> MSLSFCGNNISSYNIYHGVLQNPCFVDALNLVPHVFLLFITFPILFIGWGSQSSKVQIHHNTWLHFPGHNLRWILTFALLFVHVCEIAEGIVSDSQRASRHLHLFMPAVMGFVATTTSIVYYHNIETSNFPKLLLALFLYWVMAFITKTIKLVKYWQLGWGMSDLRFCITGVMVILNGLLMAVEINVIRVRRYVFFMNPQKVKPPEDLQDLGVRFLQPFVNLLSKATYWWMNTLIISAHRKPIDLKAIGKLPIAMRAVTNYVCLKEAYEEQKKKAADHPNRTPSIWLAMYRAFGRPILLSSTFRYLADLLGFAGPLCISGIVQRVNEPKNNTTRFSETLSSKEFLENAHVLAVLLFLALILQRTFLQASYYVTIETGINLRGALLAMIYNKILRLSTSNLSMGEMTLGQINNLVAIETNQLMWFLFLCPNLWAMPVQIIMGVILLYNLLGSSALVGAAVIVLLAPIQYFIATKLAEAQKSTLDYSTERLKKTNEILKGIKLLKLYAWEHIFCKSVEETRMKELSSLKTFALYTSLSIFMNAAIPIAAVLATFVTHAYASGNNLKPAEAFASLSLFHILVTPLFLLSTVVRFAVKAIISVQKLNEFLLSDEIGEDSWRTGEGTLPFESCKKHTGVQSKPINRKQPGRYHLDNYEQARRLRPAETEDVAIKVTNGYFSWGSGLATLSNIDIRIPTGQLTMIVGQVGCGKSSLLLAILGEMQTLEGKVYWNNVNESEPSFEATRSRSRYSVAYAAQKPWLLNATVEENITFGSSFNRQRYKAVTDACSLQPDIDLLPFGDQTEIGERGINLSGGQRQRICVARALYQNTNIVFLDDPFSALDIHLSDHLMQEGILKFLQDDKRTVVLVTHKLQYLTHADWIIAMKDGSVLREGTLKDIQTKDVELYEHWKTLMNRQDQELEKDMEADQTTLERKTLRRAMYSREAKAQMEDEDEEEEEEEDEDDNMSTVMRLRTKMPWKTCWWYLTSGGFFLLFLMIFSKLLKHSVIVAIDYWLATWTSEYSINDPGKADQTFYVAGFSILCGAGIFLCLVTSLTVEWMGLTAAKNLHHNLLNKIILGPIRFFDTTPLGLILNRFSADTNIIDQHIPPTLESLTRSTLLCLSAIGMISYATP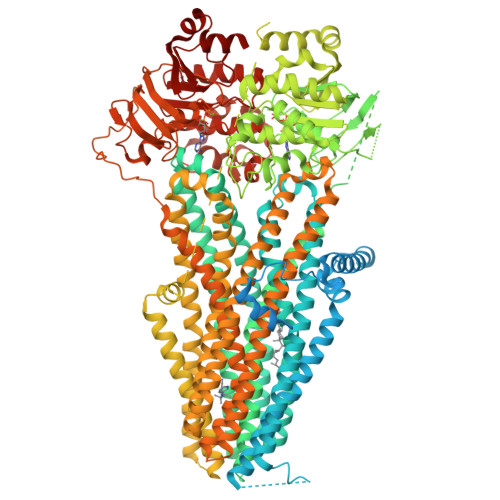VFLIALAPLGVAFYFIQKYFRVASKDLQELDDSTQLPLLCHFSETAEGLTTIRAFRHETRFKQRMLELTDTNNIAYLFLSAANRWLEVRTDYLGACIVLTASIASISGSSNSGLVGLGLLYALTITNYLNWVVRNLADLEVQMGAVKKVNSFLTMESENYEGTMDPSQVPEHWPQEGEIKIHDLCVRYENNLKPVLKHVKAYIKPGQKVGICGRTGSGKSSLSLAFFRMVDIFDGKIVIDGIDISKLPLHTLRSRLSIILQDPILFSGSIRFNLDPECKCTDDRLWEALEIAQLKNMVKSLPGGLDATVTEGGENFSVGQRQLFCLARAFVRKSSILIMDEATASIDMATENILQKVVMTAFADRTVVTIAHRVSSIMDAGLVLVFSEGILVECDTGPNLLQHKNGLFSTLVMTNK>[4x]AKVRIYQLAKELGM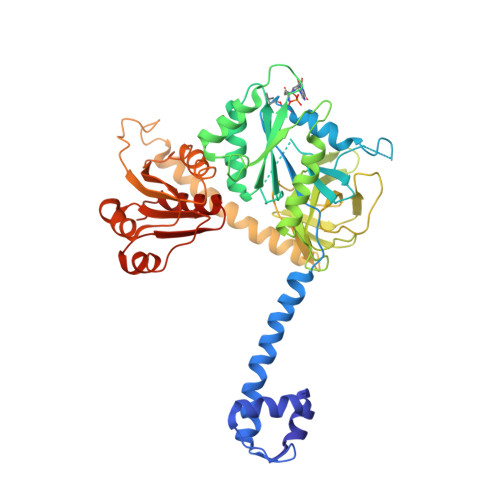ECQELLELLDQMGVAYKSHASTLEEKDAEAVRELVKEQRGLQEKLAEEERRKSLPRRPPVVVIMGHVDHGKTTLLDYLRKSRIAEKEAGGITQHVGAFEVKTPQGTVVFIDTPGHEAFTTIRQRGAKVADIAVIVIAADDGIMPQTEEAIAHAKAAGAKLIFAINKIDLPQADPEKVKRQLMERGFVPEEYGGDAIVIPISAKTGQGVQDLLEMILLLAELEDYRADPNAEPRGVILESKLDKQAGIIANMLVQEGTFRVGDYVVAGEAYGRIRAMMDADGNQRKEAGPGSAVQVLGFQELPHPGDVVEWVPDLEAAKEIAEERKEERKAREEEEKARRPRTMAELLRAMQEEGRKELNLILRADTQGSLEAIQHILARESTEDVKINILLAQVGAPTESDVLLAQTANAAILAFGVNPPGSVKKKAEEKGVLLKTFRIIYDLVDEVRNMVKGQREPQY> MASVHGTTYELLRRQGIDTVFGNPGSNELPFLKDFPEDFRYILALQEACVVGIADGYAQASRKPAFINLHSAAGTGNAMGALSNAWNSHSPLIVTAGQQTRAMIGVEALLTNVDAANLPRPLVKWSYEPASAAEVPHAMSRAIHMASMAPQGPVYLSVPYDDWDKDADPQSHHLFDRHVSSSVRLNDQDLDILVKALNSASNPAIVLGPDVDAANANADCVMLAERLKAPVWVAPSAPRCPFPTRHPCFRGLMPAGIAAISQLLEGHDVVLVIGAPVFRYHQYDPGQYLKPGTRLISV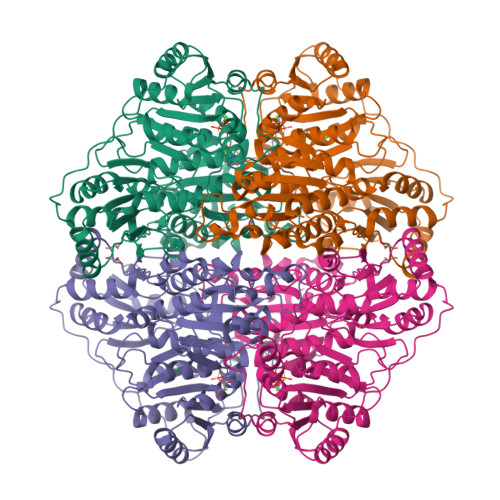TCDPLEAARAPMGDAIVADIGAMASALANLVEESSRQLPTAAPEPAKVDQDAGRLHPETVFDTLNDMAPENAIYLNESTSTTAQMWQRLNMRNPGSYYFCAAGGIGFALPAAIGVQLAEPERQVIAVIGDGSANYSISALWTAAQYNIPTIFVIMNNGTYGALRWFAGVLEAENVPGLDVPGIDFRALAKGYGVQALKADNLEQLKGSLQEALSAKGPVLIEVSTVSPVKRSHHHHHH> EAPHLVQVDAARALWPLRRFWRS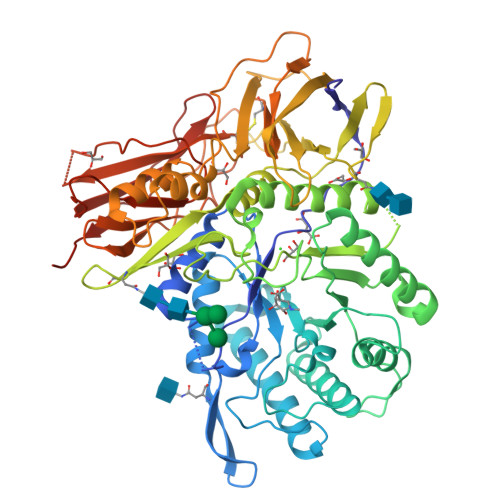TGFCPPLPHSQADPYVLSWDQQLNLAYVGAVPHRGIKQVRTHWLLELVTTRGSTGRGLSYNFTHLDGYLDLLRENQLLPGFELMGSASGHFTDFEDKQQVFEWKDLVSSLARRYIGRYGLAHVSKWNFETWNEPDHHDFDNVSMTMQGFLNYYDACSEGLRAASPALRLGGPGDSFHTPPRSPLSWGLLRHCHDGTNFFTGEAGVRLDYISLHRKGARSSISILEQEKVVAQQIRQLFPKFADTPIYNDEADPLVGWSLPQPWRADVTYAAMVVKVIAQHQNLLLANTTSAFPYALLSNDNAFLSYHPHPFAQRTLTARFQVNNTRPPHVQLLRKPVLTAMGLLALLDEEQLWAEVSQAGTVLDSNHTVGVLASAHRPQGPADAWRAAVLIYASDDTRAHPNRSVAVTLRLRGVPPGPGLVYVTRYLDNGLCSPDGEWRRLGRPVFPTAEQFRRMRAAEDPVAAAPRPLPAGGRLTLRPALRLPSLLLVHVCARPEKPPGQVTRLRALPLTQGQLVLVWSDEHVGSKCLWTYEIQFSQDGKAYTPVSRKPSTFNLFVFSPDTGAVSGSYRVRALDYWARPGPFSDPVPYLEVPVPRGPPSPGNP;> EAPHLVQVDAARALWPLRRFWRSTGFCPPLPHSQADPYVLSWDQQLNLAYVGAVPHRGIKQVRTHWLLELVTTRGSTGQGLSYNFTHLDGYLDLLRENQLLPGFELMGSASGHFTDFEDKQQVFEWKDLVSSLARRYIGRYGLAHVSKWNFETWNEPDHHDFDNVSMTMQGFLNYYDACSEGLRAASPALRLGGPGDSFHTPPRSPLSWGLLRHCHDGTNFFTGEAGVRLDYISLHRKGARSSISILEQEKVVAQQIRQLFPKFADTPIYNDEADPLVGWSLPQPWRADVTYAAMVVKVIAQHQNLLLANTTSAFPYALLSNDNAFLSYHPHPFAQRTLTARFQVNNTRPPHVQLLRKPVLTAMGLLALLDEEQLWAEVSQAGTVLDSNHTVGVLASAHRPQGPADAWRAAVLIYASDDTRAHPNRSVAVTLRLRGVPPGPGLVYVTRYLDNGLCSPDGEWRRLGRPVFPTAEQFRRMRAAEDPVAAAPRPLPAGGRLTLRPALRLPSLLLVHVCARPEKPPGQVTRLRALPLTQGQLVLVWSDEHVGSKCLWTYEIQFSQDGKAYTPVSRKPSTFNLFVFSPDTGAVSGSYRVRALDYWARPGPFSDPVPYLEVPVPRGPPSPGNP>AECSVDIQGNDQMQWNTNAITVDKSCKQFTVNLSHPGNLPKNVMGHNFVLSTAADMQGVVTDGMASGLDKDFLKPDDSRVIAQTKLIGSGEKDSVTFDVSKLKEGEQFMF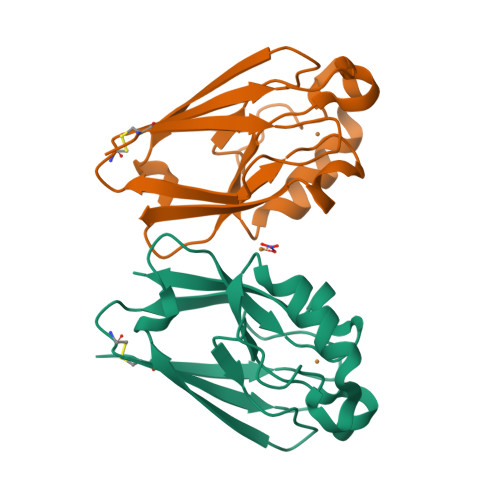FCTFPGHSALMKGHLTLK[2x]>[3x]MKTIKDRIAKWSAIGLLSAVAATAFYAPSASAHGEKSQAAFMRMRTIHWYDLSWSKEKVKINETVEIKGKFHVFEGWPETVDEPDVAFLNVGMPGPVFIRKESYIGGQLVPRSVRLEIGKTYDFRVVLKARRPGDWHVHTMMNVQGGGPIIGPGKWITVEGSMSEFRNPVTTLTGQTVDLENYNEGNTYFWHAFWFAIGVAWIGYWSRRPIFIPRLLMVDAGRADELVSATDRKVAMGFLAATILIVVMAMSSANSKYPITIPLQAGTMRGMKPLELPAPTVSVKVEDATYRVPGRAMRMKLTITNHGNSPIRLGEFYTASVRFLDSDVYKDTTGYP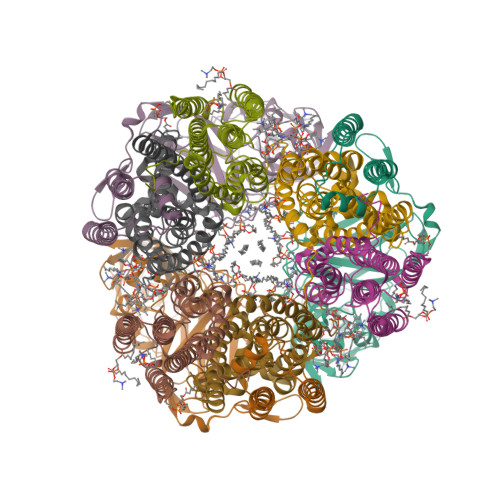EDLLAEDGLSVSDNSPLAPGETRTVDVTASDAAWEVYRLSDIIYDPDSRFAGLLFFFDATGNRQVVQIDAPLIPSFM;>[3x]MSAAQSAVRSHAEAVQVSRTIDWMALFVVFFVIVGSYHIHAMLTMGDWDFWSDWKDRRLWVTVTPIVLVTFPAAVQSYLWERYRLPWGATVCVLGLLLGEWINRYFNFWGWTYFPINFVFPASLVPGAIILDTVLMLSGSYLFTAIVGAMGWGLIFYPGNWPIIAPLHVPVEYNGMLMSIADIQGYNYVRTGTPEYIRMVEKGTLRTFGKDVAPVSAFFSAFMSILIYFMWHFIGRWFSNERFLQST;>MAATTIGGAAAAEAPLLDKKWLTFALAIYTVFYLWVRWYEGVYGWSAGLDSFAPEFETYWMNFLYTEIVLEIVTASILWGYLWKTRDRNLAALTPREELRRNFTHLVWLVAYAWAIYWGASYFTEQDGTWHQTIVRDTDFTPSHIIEFYLSYPIYIITGFAAFIYAKTRLPFFAKGISLPYLVLVVGPFMILPNVGLNEWGHTFWFMEELFVAPLHYGFVIFGWLALAVMGTLTQTFYSFAQGGLGQSLCEAVDEGLIAK[3x]>[4x]SEEVVIAGMSGKLPESENLQEFWANLIGGVDMVTDDDRRWKAGLYGLPKRSGKLKDLSKFDASFFGVHPKQAHTMDPQLRLLLEVSYEAIVDGGINPASLRGTNTGVWVGVSGSEASEALSRDPETLLGYSMVGCQRAMMANRLSFFFDFKGPSIALDTACSSSLLALQNAYQAIRSGECPAALVGGINLLLKPNTSVQFMKLGMLSPDGTCRSFDDSGSGYCRSEAVVAVLLTKKSLARRVYATILNAGTNTDGSKEQGVTFPSGEVQEQLICSLYQPAGLAPESLEYIEAHGTGTKVGDPQELNGITRSLCAFRQAPLLIGSTKSNMGHPEPASGLAALTKVLLSLEHGVWAPNLHFHNPNPEIPALLDGRLQVVDRPLPVRGGNVGI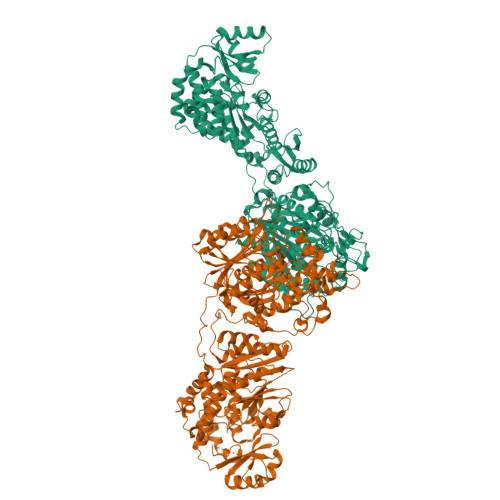NSFGFGGSNVHVILQPNTRQAPAPTAHAALPHLLHASGRTLEAVQDLLEQGRQHSQDLAFVSMLNDIAATPTAAMPFRGYTVLGVEGRVQEVQQVSTNKRPLWFICSGMGTQWRGMGLSLMRLDSFRESILRSDEAVKPLGVKVSDLLLSTDERTFDDIVHAFVSLTAIQIALIDLLTSVGLKPDGIIGHSLGEVACGYADGCLSQREAVLAAYWRGQCIKDAHLPPGSMAAVGLSWEECKQRCPAGVVPACHNSEDTVTISGPQAAVNEFVEQLKQEGVFAKEVRTGGLAFHSYFMEGIAPTLLQALKKVIREPRPRSARWLSTSIPEAQWQSSLARTSSAEYNVNNLVSPVLFQEALWHIPEHAVVLEIAPHALLQAVLKRGVKSSCTIIPLMKRDHKDNLEFFLTNLGKVHLTGINVNPNALFPPVEFPAPRGTPLISPHIKWDHSQTWDVPVAEDFPN> GMEPIMRNPEDALLDSWHQNAQAWIDAVRHGAIESRRQVTDQAILLAILGRQPERVLDLGCGEGWLLRALADRGIEAVGVDGDRTLVDAARAAGAGEVHLASYAQLAEAKVPVGKDYDLICANFALL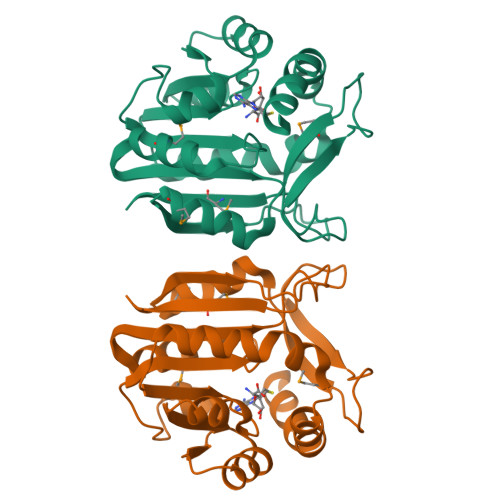HQDIIELLSAMRTLLVPGGALVIQTLHPWSVADGDYQDGWREESFAGFAGDWQPMPWYFRTLASWLNALDMAGLRLVSLQEPQHPQSAVPQSLLMVAERH> GPGSGKNKVRRVKTIYDCQADNDDELTFIEGEVIIVTGEEDQEWWIGHIEGQPERKGVFPVSFV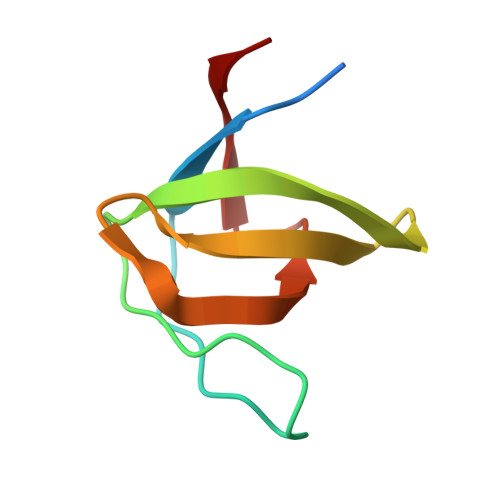HILSD> MTTQLRYENNDDDERVEYNLFTNRSTMMANFEEWIKMATDNKINSRNSWNFALIDYFYDLDVLKDGENNINFQKASATLDGCIKIYSSRVDSVTTETGKLLSGLAQRKTNGASNGDDSNGGNGEGLGGDSDEANIEIDPLTGMPISNDPDVNNTRRRVYNRVLETTLVEFETIKMKELDQELIIDPLFKKALVDFDEGGAKSLLLNTLNIDNTARVIFDASIKDTQNVGQGKLQRKEEELIERDSLVDDENEPSQSLISTRNDSTVNDSVISAPSMEDEILSLGMDFIKFDQIAVCEISGSIEQLRNVVEDINQAKDFIENVNNRFDNFLTEEELQAAVPDNAEDDSDGFDMGMQQELCYPDENHDNTSHDEQDDDNVNSTTGSIFEKDLMAYFDENLNRNWRGREHWKVRNFKKANLVNKESDLLEETRTTIGDTTDKNTTDDKSMDTKKKHKQKKVLEIDFFKTDDSFEDKVFASKGRTKIDMPIKNRKNDTHYLLPDDFHFSTDRITRLFIKPGQKMSLFSHRKHTRGDVSSGLFEKSTVSANHSNNDIPTIADEHFWADNYERKEQEEKEKEQSKEVGDVVGGALDNPFEDDMDGVDFNQAFEGTDDNEEASVKLDLQDDEDHKFPIRENKVTYSRVSKKVDVRRLKKNVWRSINNLIQEHDSRKNREQSSNDSETHTEDESTKELKFSDIIQGISKMYSDDTLKDISTSFCFICLLHLANEHGLQITHTENYNDLIVNYEDLATTQAAS;> MQDPDGIDINTKIFNSVAEVFQKAQGSYAGHRKHIAVLKKIQSKAVEQGYEDAFNFWFDKLVTKILPLKKNEIIGDRIVKLVAAFIASLERELILAKKQNYKLTNDEEGIFSRFVDQFIRHVLRGVESPDKNVRFRVLQLLAVIMDNIGEIDESLFNLLILSLNKRIYDREPTVRIQAVFCLTKFQDEEQTEHLTELSDNEENFEATRTLVASIQNDPSAEVRRAAMLNLINDNNTRPYILERARDVNIVNRRLVYSRILKSMGRKCFDDIEPHIFDQLIEWGLEDRELSVRNACKRLIAHDWLNALDGDLIELLEKLDVSRSSVCVKAIEALFQSRPDILSKIKFPESIWKDFTVEIAFLFRAIYLYCLDNNITEMLEENFPEASKLSEHLNHYILLRYHHNDISNDSQSHFDYNTLEFIIEQLSIAAERYDYSDEVGRRSMLTVVRNMLALTTLSEPLIKIGIRVMKSLSINEKDFVTMAIEIINDIRDDDIEKQEQEEKIKSKKINRRNETSVDEEDENGTHNDEVNEDEEDDNISSFHSAVENLVQGNGNVSESDIINNLPPEKEASSATIVLCLTRSSYMLELVNTPLTENILIASLMDTLITPAVRNTAPNIRELGVKNLGLCCLLDVKLAIDNMYILGMCVSKGNASLKYIALQVIVDIFSVHGNTVVDGEGKVDSISLHKIFYKVLKNNGLPECQVIAAEGLCKLFLADVFTDDDLFETLVLSYFSPINSSNEALVQAFAFCIPVYCFSHPAHQQRMSRTAADILLRLCVLWDDLQSSVIPEVDREAMLKPNIIFQQLLFWTDPRNLVNQTGSTKKDTVQLTFLIDVLKIYAQIEKKEIKKMIITNINAIFLSSEQDYSTLKELLEYSDDIAENDNLDNVSKNALDKLRNNLNSLIEEINERSETQTKDENNTANDQYSSILGNSFNKSSNDTIEHAADITDGNNTELTKTTVNISAVDNTTEQSNSRKRTRSEAEQIDTSKNLENMSIQDTSTVAKNVSFVLPDEKSDAMSIDEEDKDSESFSEVC

DNA needs to be compacted to fit into nuclei and during cell division, when dense chromatids are formed for their mechanical segregation, a process that depends on the protein complex condensin. It forms and enlarges loops in DNA through loop extrusion. The core SMC complex is a heterotrimeric ring consisting of two SMC proteins and a kleisin, and in condensin these are Smc2, Smc4, and Brn1, respectively. To complete condensin, two HEAT repeat-containing proteins Associated With Kleisins (HAWKs), Ycs4 and Ycg1, stably bind to central regions of Brn1.

To determine whether Ycg1 also interacts with the head module in the DNA-bound, clamped state we mixed the condensin pentamer with 80-bp DNA, ADP, and BeF3 as before and examined by cryo-EM. Second, from the same dataset, we solved the structure of Ycg1 bound to DNA at 3.2-Å resolution. In this structure, the region of Brn1 that binds Ycg1 and makes up the “safety belt” (residues 387 to 524) was mostly resolved, with the exception of a disordered connecting loop (residues 411 to 458). The DNA is somewhat bent as it passes over the DNA-binding surface of Ycg1 and through the safety belt. The DNA covers most of Ycg1’s positively charged surface, and we could identify more Ycg1–DNA interactions than a previous study using X-ray crystallography, which used a shorter DNA. The fact that we observed Ycg1 bound to Brn1 while not being bound to the head module of condensin strongly suggests that in condensin’s clamped state Ycg1 remains attached to the rest of the complex via the flexible linkers provided by Brn1 either side of its interaction site with Ycg1. The next resolved Brn1 residues bind to Ycg1 and form the safety belt around DNA (Brn1: 459 to 525), before Brn1’s C-terminal winged-helix domain binds to the cap of Smc4 (Brn1: 526 to 747). Our cryo-EM data provide clear evidence that condensin can bind to DNA via Ycg1 and the clamped head module simultaneously. Based on our structures and published single-molecule experiments we propose that this is an intermediate step in the loop extrusion process and the variable distance of Ycg1 with respect to the head module might determine or allow condensin to make steps on DNA that are needed to extrude loops and to enlarge them. In this scenario, Ycg1 is likely to act as a static anchor on the DNA, which implies that the clamped DNA is being translocated during loop extrusion, consistent with the regulation of DNA clamping by ATP turnover.>MKAIDKMTDNPPQEGLSGRKIIYDEDGKPSRSCNTLLDFQYVTGKISNGLKNLSSNGKLAGTGALTGEASELMPGSRTYRKVDPPDVEQLGRSSWTLLHSVAASYPAQPTDQQKGEMKQFLNIFSHIYPCNWSAKDFEKYIRENAPQVESREELGRWMCEAHNKVNKKLRKPKFDCNFWEKRWKDG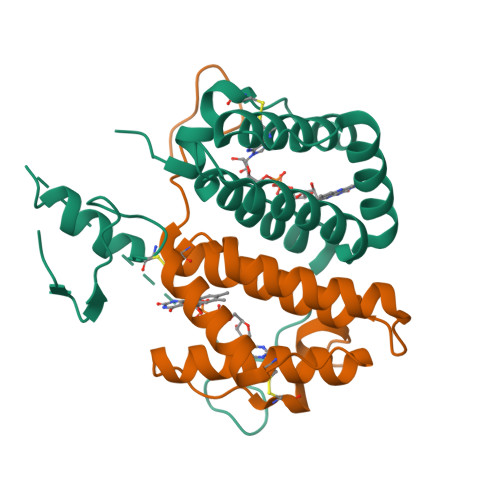WDE[3x]>[4x]MEYRYDDNATNVKAMKYLIEHYFDNFKVDSIEIIGSGYDSVAYLVNNEYIFKTKFSTNKKKGYAKEKAIYNFLN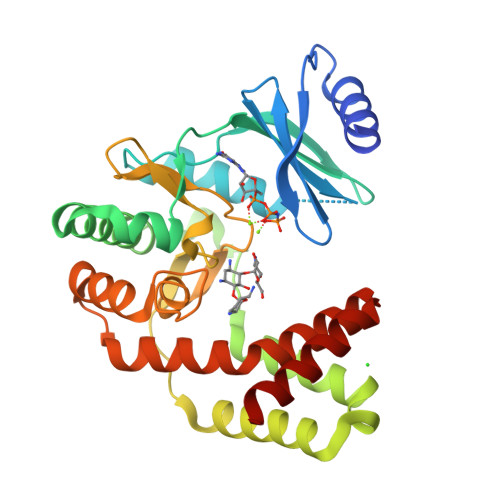TNLETNVKIPNIEYSYISDELSILGYKEIKGTFLTPEIYSTMSEEEQNLLKRDIASFLRQMHGLDYTDISECTIDNKQNVLEEYILLRETIYNDLTDIEKDYIESFMERLNATTVFEGKKCLCHNDFSCNHLLLDGNNRLTGIIDFGDSGIIDEYCDFIYLLEDSEEEIGTNFGEDILRMYGNIDIEKAKEYQDIVEEYYPIETIVYGIKNIKQEFIENGRKEIYKRTYKD> MRRVSFSVVLATFGKRHSSIFSPRYDWRTSGVHDIAPRDEGDFLYQGPQHVLPGAHPLPLHHPHNTITRPVISPYIPSPQRSHPYFTAPLPELPHFSTTKPIVYTYGTMKERIIAPVFNLKNEVIYTRELDPFIFGMYPEVEELSKNLTYWMVRCQNFASKWDYETREIWRKAKKNWPNTGMGMPRVGNRKNHLYTWGGRTKPSKPWNMLMPTMDVKTWSKSNRMMLTLKMLQGRLQVVDRLTLEEPTQECYLELCRNMSWDVRHTGGGVLFMDGGSRITPSSEFDRAFFFGSFFNGRNKIVRPTVLCDEQYDYNKTAAKQRMKGPKGAKNPIPINRFNAYDAMKHDRLVITEGALMQLEDELYEHKLQILPPHIRNQLPEYGYLDSEALGDCVPSL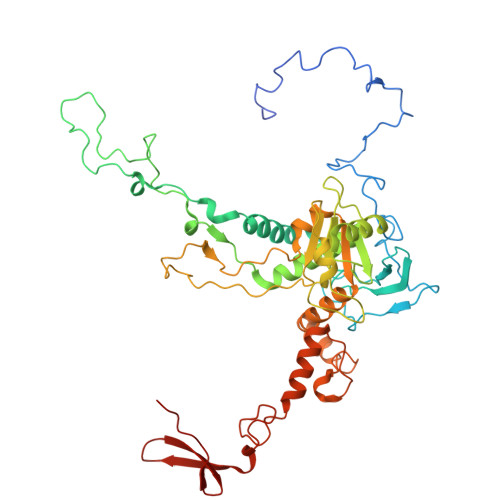KTIQMEAAARTEEAESDMYKSFIDNPYNPWKDNMDASYAVDGADGTVQKFVDGKKVSWSMLS>[2x]FPTIPLSRLA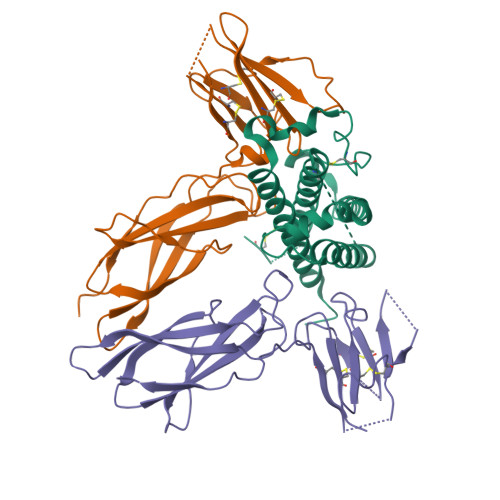DNAWLRADRLNQLAFDTYQEFEEAYIPKEQIHSFWWNPQTSLCPSESIPTPSNKEETQQKSNLELLRISLLLIQSWLEPVQFLRSVFANSLVYGASDSNVYDLLKDLEEGIQTLMGRLEDGSPRTGQIFKQTYSKFDTNSHNDDALLKNYGLLYCFNKDMSKVSTYLRTVQCRSVEGSCGF;>[4x]FSGSEATAAILSRAPWSLQSVNPGLKTNSSKEPKFTKCRSPERETFSCHWTDEVHHGTKNLGPIQLFYTRRNTQEWTQEWKECPDYVSAGENSCYFNSSFTSIWIPYCIKLTSNGGTVDEKCFSVDEIVQPDPPIALNWTLLNVSLTGIHADIQVRWEAPRNADIQKGWMVLEYELQYKEVNETKWKMMDPILTTSVPVYSLKVDKEYEVRVRSKQRNSGNYGEFSEVLYVTLPQMSQ PHOSPHOSERINE | C3 H8 N O6 P | 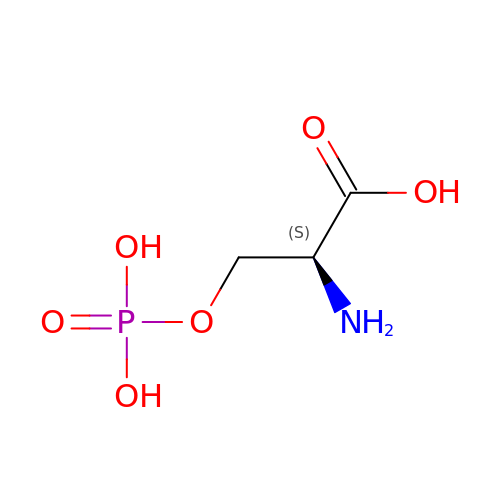BZQFBWGGLXLEPQ-REOHCLBHSA-N Transcription activator-like (TAL) effectors specifically bind to double stranded (ds) DNA through a central domain of tandem repeats. Each TAL effector (TALE) repeat comprises 33–35 amino acids and recognizes one specific DNA base through a highly variable residue at a fixed position in the repeat. The crystal structures of TAL effector (TALE) proteins bound to their respective target DNAs have revealed that the residue at position 13 is the only one directly involved in DNA base recognition, whereas the 12th residue stabilizes the proper loop conformation. dHax3, an engineered TALE protein, proved to be a useful scaffold for structural characterizations. We then present fifteen crystal structures of engineered dHax3 variants in complex with target DNA molecules, which elucidate the structural basis for the recognition of bases adenine (A) and guanine (G) by reported or uncharacterized TALE codes.

The structural observation suggests that Ile34 may not be a major contributor to the affinity of DNA binding by TALE repeats, consistent with the classification of NI as a “weak” TALE code. It also insinuates that base A may “tolerate” a wide range of amino acids at position 34 of a TALE repeat when there is no steric clash. To test this speculation, we generated dHax3 variants with the 34th residue on repeat 7 substituted with different amino acids. In total, we obtained nine high-quality structures that elucidate the accommodation of base A by Leu, Met, Cys, Pro, Trp, His, Thr, Asn, and Glu at the 34th position. Among these, the hydrophobic residues Leu, Met, Cys, and Pro all adopt conformations that do not clash with base A. As what happens to Ile34, there is no specific coordination found between these hydrophobic residues and base A. Trp, Thr, and His, in spite of the presence of polar groups, do not form H-bond with base A. They also appear to adopt conformations that simply avoid steric clash. These residues may all represent weak code, if they are used for base recognition.

>[2x]MQWSGARALEALLTVAGELRGPPLQLDTGQLLKIAKRGGVTAVEAVHAWRNALTGAPLNLTPEQVVAIASHDGGKQALETVQRLLPVLCQAHGLTPQQVVAIASHDGGKQALETVQRLLPVLCQAHGLTPEQVVAIASHDGGKQALETVQALLPVLCQAHGLTPEQVVAIASNGGGKQALETVQRLLPVLCQAHGLTPQQVVAIASNGGGKQALETVQRLLPVLCQAHGLTPQQVVAIASNGGGKQALETVQRLLPVLCQAHGLTPQQVVAIASNTGGKQALETVQRLLPVLCQAHGLTPQQVVAIASNGGGKQALETVQRLLPVLCQAHGLTPQQVVAIASHDGGKQALETVQRLLPVLCQAHGLTPEQVVAIASNGGGKQALETVQRLLPVLCQAHGLTPEQVVAIASHDGGKQALETVQRLLPVLCQAHGLTPQQVVAIASNGGGRPALESIVAQLSRPDPALAALTNDHLVALACLGGRPALDAVKKLEHHHHHH>[4x]MARKYFVAANWKCNGTLESIKSLTNSFNNLDFDPSKLDVV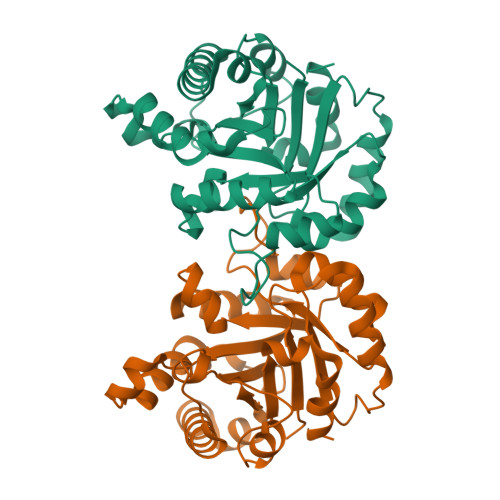VFPVSVHYDHTRKLLQSKFSTGIQNVSKFGNGSYTGEVSAEIAKDLNIEYVIIGHFERRKYFHETDEDVREKLQASLKNNLKAVVCFGESLEQREQNKTIEVITKQVKAFVDLIDNFDNVILVYEPLFAIGTGKTATPEQAQLVHKEIRKIVKDTCGEKQANQIRILYGGSVNTENCSSLIQQEDIDGFLVGNASLKESFVDIIKSAM>YFQSMEPKVAELKQKIEDTLCPFGFEVYPFQ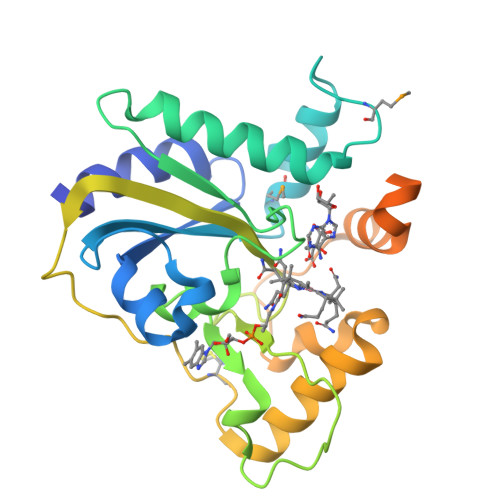VAWYNELLPPAFHLPLPGPTLAFLVLSTPAMFDRALKPFLQSCHLRMLTDPVDQCVAYHLGRVRESLPELQIEIIADYEVHPNRRPKILAQTAAHVAGAAYYYQRQDVEADPWGNQRISGVCIHPRFGGWFAIRGVVLLPGIEVPDLPPRKPHDCVPTRADRIALLEGFNFHWRDWTYRDAVTPQERYSEEQKAYFSTPPAQRLALLGLAQPSEKPSSPSPDLPFTTPAPKKPGNPSRARSWLSPRVSPPASPGP[16x]>MALSDRLELVSASEIRKLFDIAAGMKDVISLGIGEPDFDTPQHIKEYAKEALDKGLTHYGPNIGLLELREAIAEKLKKQNGIEADPKTEIMVLLGANQAFLMGLSAFLKDGEEVLIPTPAFVSYAPAVILAGGKPVEVPTYEEDEFRLNVDELKKYVTDKTRALIINSPCNPTGAVLTKKDLEEIADFVVEHDLIVISDEVYEHFIYDDARHYSIASLDGMFERTITVNGFSKTFAMTGWRLGFVAAPSWIIERMVKFQMYNATCPVTFIQYAAAKALKDERSWKAVEEMRKEYD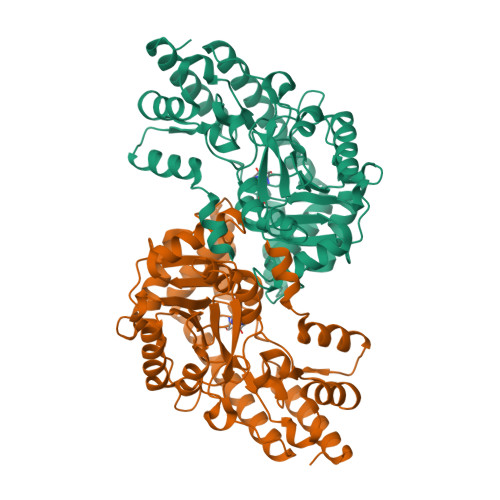RRRKLVWKRLNEMGLPTVKPKGAFYIFPRIRDTGLTSKKFSELMLKEARVAVVPGSAFGKAGEGYVRISYATAYEKLEEAMDRMERVLKERKLV[2x]> GMAKATTIKDAIRIFEERKSVVATEAEKVELHGMIPPIEKMDATLSTLKACKHLALSTNNIEKISSLSGMENLRILSLGRNLIKKIENLDAVADTLEELWISYNQIASLSGIEKLVNLRVLYMSNNKITNWGEIDKLAALDKLEDLLLAGNPLYNDYKENNATSEYRIEVVKRLPNLK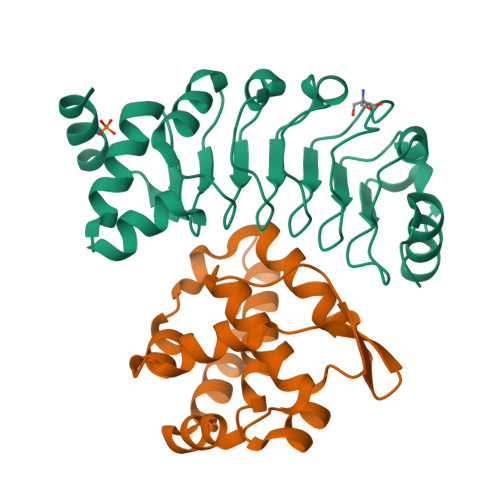KLDGMPVDVDEREQANVARGG;> GDLAAAKPALDAALEALNSIKDGDIKNLKALKKPPQIITRIFDCVLVLRMLPVTKAEYTDEKGRMVQVGNYPEAQKMMNQMSFLQDLKDFAKEQINDETVELLEPYFMSEDFTFENAQKASGNVAGLCNWAESMAKYHNVAKVVE N-(2-phenylethyl)thioformamide | C9 H11 N S | 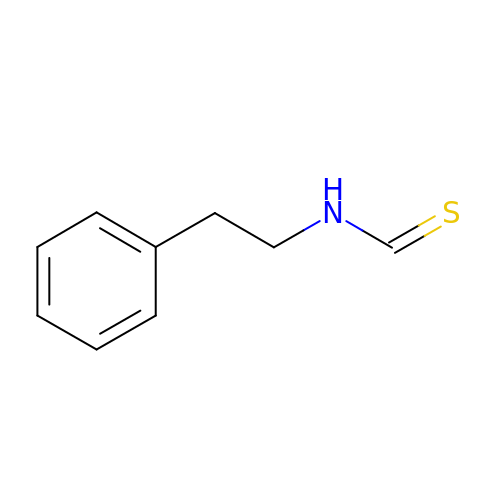WVJCPUDEWCGDGL-UHFFFAOYSA-N>GAMDPRTITMHKDSTGHVGFIFKNGKITSIVKDSSAARNGLLTEHNICEING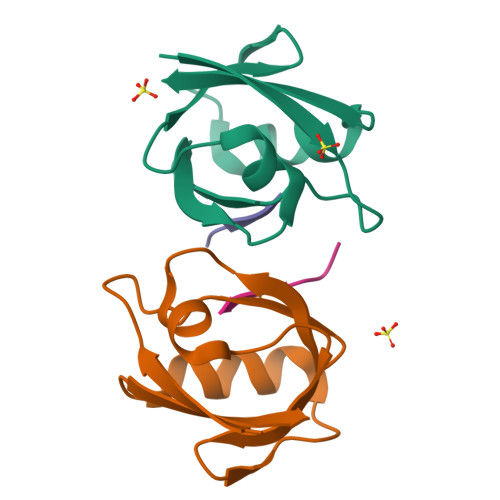QNVIGLKDSQIADILSTSGTVVTITIM[2x];>TNEFYA[2x]>MPQAFFSHNNKDKKIVLEVLEHLRQSLVATWIDQQSIPGGGSLIQQIIAGISKSQYFLAFLSNEYLKSDWCWDELEQAYALHQKGKVKIIPILLTNRAQLDLNALTDARRNFLESILTRLKYVEFDPHNMTRSLGSVAEALWQNEAVRFEPIRMIKVNGTELQVVEFKIPGSNLPVDFLHHWDLKIEDFIATSPNEQKPVKFDVPVALYGPGPNWLYAFLTLPFKNRNTVFVFNSRTSEYICVYSKSAGLAPGMVLKGHHHHH[30x]

Here we investigated a protein containing a CARF domain fused Toll/interleukin-1 receptor (TIR) domain, Cat1. We found that Cat1 provides immunity by cleaving and depleting NAD+ molecules from the infected host, inducing a growth arrest that prevents viral propagation. Cat1 forms dimers that stack upon each other to generate long filaments that are maintained by bound cOA ligands, with stacked TIR domains forming the NAD+ cleavage catalytic sites. Further, Cat1 filaments assemble into unique trigonal and pentagonal networks that enhance NAD+ degradation.

The cryo-EM structure of cA4-bound Cat1 shows that the complex assembles into filamentous structures, forming intricate higher-order networks. To our surprise, we observed that the trigonal filament assembly further associates with more Cat1 filaments generating a pentameric assembly. In the cryo-EM 3D classification, we observed two distinct classes, one corresponds to the trigonal filament bundle, described previously, and the other where five trigonal filament bundles join to form a large pentameric assembly. The inter-repeat unit interaction between β1β2- loop on both sides of a dimeric CARF domain of a Cat1 dimer and the TIR domain of the adjacent Cat1 dimer, enables the assembly extension and provides an opportunity to form an even larger filament network. As the filament network spreads, flexibility results in broken densities (marked as “1” in black dashed lines), preventing model building for these segments. The tilt of the third Cat1 dimer around the center of the repeat unit of the trigonal filament bundle shifts the TIR domain, which points opposite to the trigonal filament assembly, above the plane with respect to the of rest of the Cat1 dimeric units of the pentameric assembly (see magenta arrow implying shift above the plane). The above-mentioned shift of the TIR domain mediates its interaction with the Cat1 dimer of the next turn and results in the generation of a closely packed spiral bundle without pitch and with a large pentagonal pore at the center. In contrast to other CARF effectors, however, the cA4 binding pocket is formed by not one but two CARF dimers, where the bottom CARF-dimer forms the base of the pocket and the top CARF dimer caps the ligand. Cryo-EM analysis of the purified proteins in the presence of cA4 demonstrated the disruption of higher order filament assembly for both mutants at 165,000 magnification, with only small filament fragments remaining. This result further supports the idea that the linear, trigonal and pentagonal filament bundles of Cat1 are not independent units, but part of the same filament network, and hence cannot be investigated on their own. In addition to the distinctive arrangement of sensor and catalytic domains, the higher-order networks formed by inter-filament association are unique to Cat1.>[2x]GAMGAWKLQTVLEKVRLSRHEISEAAEVVNWVVEHLLRRLQGGESEFKGVALLRTGSYYERVKISAPNEFDVMFKLEVPRIQLEEYCNSGAHYFVKFKRNPGGNPLEQFLEKEILSASKMLSKFRKIIKEEIKNIEDTGVTVERKRRGSPAVTLLISKPKEISVDIILALESKSSWPASTQKGLPISQWLGAKVKNNLKRQPFYLVPKHAKEGSGFQEETWRLSFSHIEKDILKNHGQSKT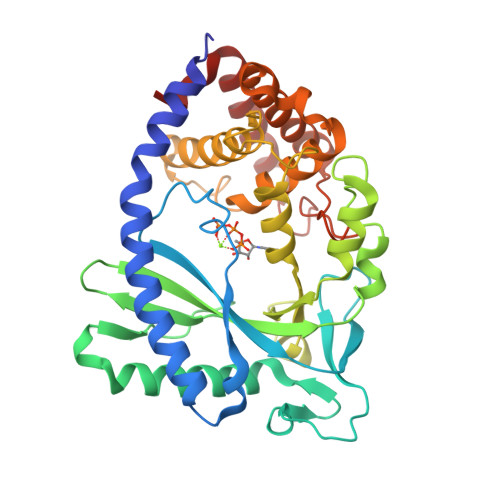CCEIDGVKCCRKECLKLMKYLLEQLKKKFGNRRELAKFCSYHVKTAFFHVCTQDPHDNQWHLKNLECCFDNCVAYFLQCLKTEQLANYFIPGVNLFSRDLIDKPSKEFLSKQIEYERNNGFPVFW>MLSPKAATLAERSAGLAFSLYQAMAKDQAVENILLSPVVVASSLGLVSLGGKATTASQAKAVLSAEQLRDEEVHAGLGELLRSLSNSTARNVTWKLGSRLYGPSSVSFAEDFVRSSKQHYNCEHSKINFRDKRSALQSINEWAAQTTDGKLPEVTKDVERTDGALLVNAMFFKPHWDEKFHHKMVDNRGFMVTRSYTVGVTMMHRTGLYNYYDDEKEKLQIVEMPLAHKLSSLIILMPHHVEPLERLEKLLTKEQLKIWMGKMQKKAVAISLPKGVVEVTHDLQKHLAGLGLTEAIDKNKADLSRMSGKKDLYLASVFHATAFEWDTEGNPFDQDIYGREELRSPKLFYADHPFIFLVRDTQSGSLLFIGRLVRPKGDKMRDELLEHHHHHH[2x];>[6x]XPPGPPGPPGPRGLPGPPGPPG

In order to function, collagens require the specific chaperone HSP47 for proper folding and secretion. Proper triple-helix formation as well as exit from the ER of procollagen molecules depends critically on HSP47, an ER-resident chaperone belonging to the serpin family. The interaction involves Gly-Xxx-Arg triplets exclusively on triple-helical procollagen. The arginine residue is located in the so-called Y0 position and forms a crucial salt bridge with an aspartic acid of HSP47 (16).

To explain this observation, we determined cocrystal structures of HSP47 with synthetic model peptides containing the GPRGFP and GPRGLP motifs (from here on called RGF and RGL, respectively). The complexes of HSP47:CMP[RGF/RGL] crystallized in space groups P3221 and I222, respectively, which both are different from those of all previously determined HSP47 crystal structures. The structures were refined at resolutions of 1.94 Å and 2.5 Å with refinement statistics of R/Rfree 20.3/24.8% and 21.3/26.7%. In contrast to all those RGP structures, these new ones employing the RGL and RGF collagen model peptides have only the A-site occupied by HSP47. To adapt the bulky hydrophobic side chains at the X+1 position, conformational rearrangements of HSP47 take place. In both structures, the loop containing His274 moves slightly outward by approximately 1.8 Å (Cα – Cα distance). The results were similar to the prediction mentioned before (RGF/B and RGL/B), the phenylalanine and—less prominently—the leucine side chain clash with either the modeled second HSP47 molecule or the collagen backbone. Still, the presence of the leucine seems to influence the positioning of the important arginine at the B-site and might prevent binding in a similar manner.> PWATAEYD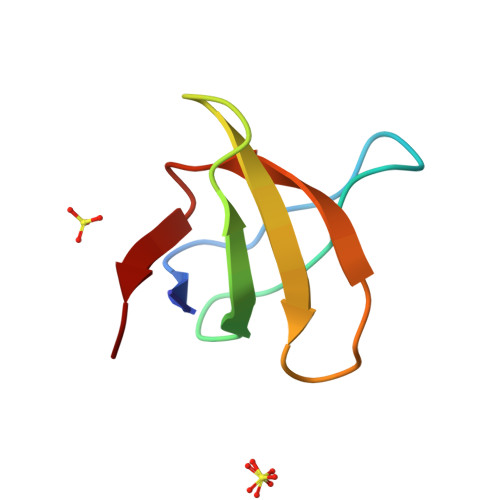YDAAEDNELTFVENDKIINIEFVDDDWWLGELEKDGSKGLFPSNYVSLGN> ANFNVPKLGVFPVAAVFDIDNVPEDSSATGSRWLPSIYQGGNYWGGGPQALHAQVSNFDSSNRLPYNPR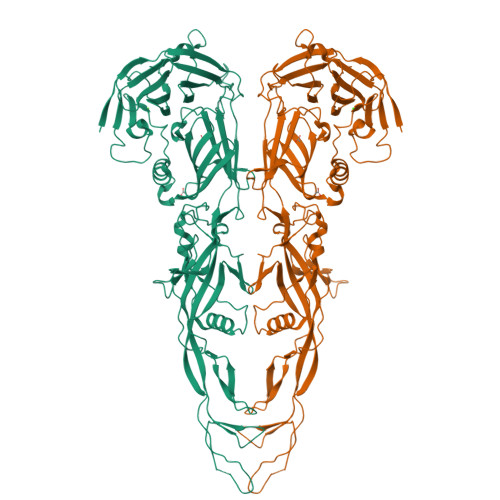TENNPAGNCAFAFNPFGQYISNISSAQSVHRRIYGIDLNDEPLFSPNAASITNGGNPTMSQDTGYHNIGPINTAYKAEIFRPVNPLPMSDTAPDPETLEPGQTEPLIKSDGVYSNSGIASFIFDRPVTEPNPNWPPLPPPVIPIIYPTPALGIGAAAAYGFGYQVTVYRWEEIPVEFIADPETCPAQPTTDKVIIRTTDLNPEGSPCAYEAGIILVRQTSNPMNAVAGRLVPYVEDIAVDIFLTGKFFTLNPPLRITNNYFADDEVKENTVTIGNYTTTLSSAYYAVYKTDGYGGATCFIASGGAGISALVQLQDNSVLDVLYYSLPLSLGGSKAAIDEWVANNCGLFPMSGGLDKTTLLEIPRRQLEAINPQDGPGQYDLFILDDSGAYASFSSFIGYPEAAYYVAGAATFMDVENPDEIIFILRNGAGWYACEIGDALKIADDEFDSVDYFAYRGGVMFIGSARYTEGGDPLPIKYRAIIPGLP>[2x]ATLTAKNLAKAYKGRRV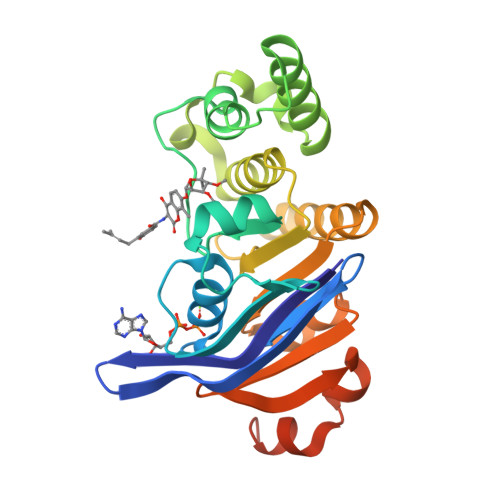VEDVSLTVNSGEIVGLLGPNGAGKTTTFYMVVGIVPRDAGNIIIDDDDISLLPLHARARRGIGYLPQEASIFRRLSVYDNLMAVLQIRDDLSAEQREDRANELMEEFHIEHLRDSMGQSLSGGERRRVEIARALAANPKFILLDEPFAGVDPISVIDIKRIIEHLRDSGLGVLITDHNVRETLAVCERAYIVSQGHLIAHGTPTEILQDEHVKRVYLGEDFRLEHHHHHHHH>EPFWADLQPRVAFVERGGSLWLNCSTNCPRPERGGLETSLRRNGTQRGLRWLARQLVDIREPETQPVCFFRCARRTLQARGLIRTFQRPDRVELMPLPPWQPVGENFTLSCRVPGAGPRASLTLTLLRGAQELIRRSFAGEPPRARGAVLTATVLARREDHGANFSCRAELDLRPHGLGLFENSSAPRELRTFSLSPDAPRLAAPRLLEVGSERPVSCTLDGLFPASEARVYLALGDQNLSPDVTLEGDAFVATATATASAEQEGARQLVCNVTLGGENRETRENVTIYSFPAPLLTLSEPSVSEGQMVTVTCAAGAQALVTLEGVPAAVPGQPAQLQLNATENDDRRSFFCDATLDVDGETLIKNRSAELRVLYAPR[2x]

ICAM-5, initially called telencephalin, is an integral type I transmembrane glycoprotein of ∼150 kDa that is expressed exclusively in telencephalic neurons. It has nine immunoglobulin superfamily (IgSF) domains, with a total of 832 amino acids in the extracellular region, a single transmembrane segment and a 64-residue cytoplasmic domain. In addition to integrin recognition shared with the other ICAMs, ICAM-5 has unique characteristics within the subfamily, as it mediates homophilic adhesion interactions that promote neurite development. The crystal structure of the four most N-terminal glycosylated domains (D1–D4) of ICAM-5 was determined in three different space groups and the D1–D5 fragment was modelled.

Comparison of the three crystal forms indicated some flexibility at the interdomain interfaces, which is probably needed to facilitate cell–cell interactions. The largest movement between the most divergent R3 and P4322 structures (r.m.s.d. of 2.7 Å) was ∼16°. The overall P21 structure is nonetheless more similar to the R3 crystal structure (5°) than to the P4322 structure (11°), even though the tetragonal and monoclinic crystals were prepared under the same conditions. This could indicate that interdomain movement depends more on crystal contacts than on crystallization conditions.>MSELEKAMVALIDVFHQYSGREGDKHKLKKSELKELINNELSHFLEEIKEQEVVDKVMETLDNDGDGECDFQEFMAFVAMVTTACHEFFEHE[2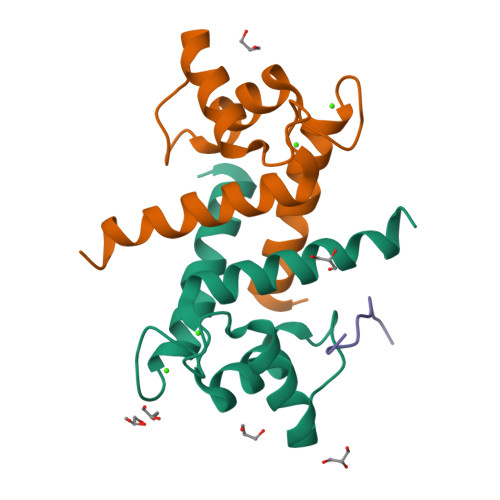x];> SPQGGGPWDSVARVL>DPSKDSKAQVSAAEAGITGTWYNQLGSTFIVTAGADGALTGTYESAVGNAESRYVLTGRYDSAPATDGSGTALGWTVAWKNNYRNAHSATTWSGQYVGGAEARINTQWLLTSGTTEANAWKSTLVGHDTF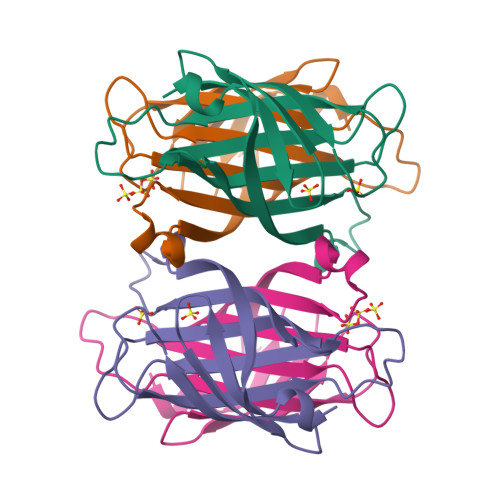TKVKP[2x]>[2x]ARPCIPKSFGYSSVVCVCNATYCDSFDPPTFPALGTFSRYESTRSGRRMELSMGPIQANHTGTGLLLTLQPEQKFQKVKGFGGAMTDAAALNILALSPPAQNLLLKSYFSEEGIGYNIIRVPMASCDFSIRTYTYADTPDDFQLHNFSLPEEDTKLKIPLIHRALQLAQRPVSLLASPWTSPTWLKTNGAVNGKGSLKGQPGDIYHQTW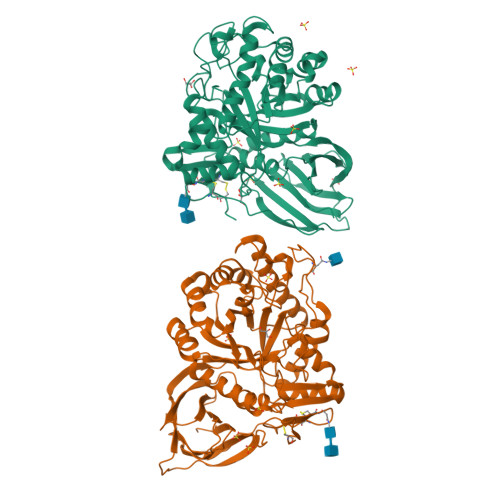ARYFVKFLDAYAEHKLQFWAVTAENEPSAGLLSGYPFQCLGFTPEHQRDFIARDLGPTLANSTHHNVRLLMLDDQRLLLPHWAKVVLTDPEAAKYVHGIAVHWYLDFLAPAKATLGETHRLFPNTMLFASEACVGSKFWEQSVRLGSWDRGMQYSHSIITSLLYHVVGWTDWNLALNPEGGPNWVRNFVDSPIIVDITKDTFYKQPMFYHLGHFSKFIPEGSQRVGLVASQKNDLDAVALMHPDGSAVVVVLNRSSKDVPLTIKDPAVGFLETISPGYSIHTYLWRRQ> GSHMRTVKVFEEAWPLHTPFVIARGSRSEARVVVVELEEEGIKGTGECTPYPRYGESDASVMAQIMSVVPQLEKGLTREELQKILPAGAARNALDCALWDLAARRQQQSLADLIGITLPETVITAQTVVIGTPDQMANSASTLWQAGAKLLKVKLDNHLISERMVA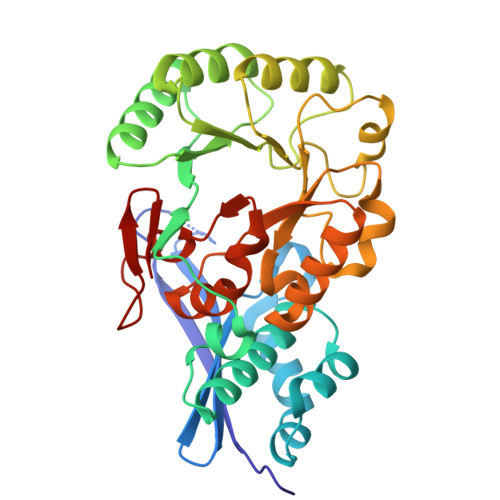IRTAVPDATLIVDANESWRAEGLAARCQLLADLGVAMLEQPLPAQDDAALENFIHPLPICADESCHTRSNLKALKGRYEMVNIKLDKTGGLTEALALATEARAQGFSLMLGCMLCTSRAISAALPLVPQVSFADLDGPTWLAVDVEPALQFTTGELHL>[30x]GAPGAPGSQGAPGLQGAPGAPGSQGAPGLQGAPGAPGSQGAPGLQGAPGAPGSQGAPGLQGAPGAPGSQGAPGLQGAPGAPGSQGAPGLQGAPGAPGSQGAPGLQGAPGAPGSQGAPGLQGAPGAPGSQGAPGLQGAPGA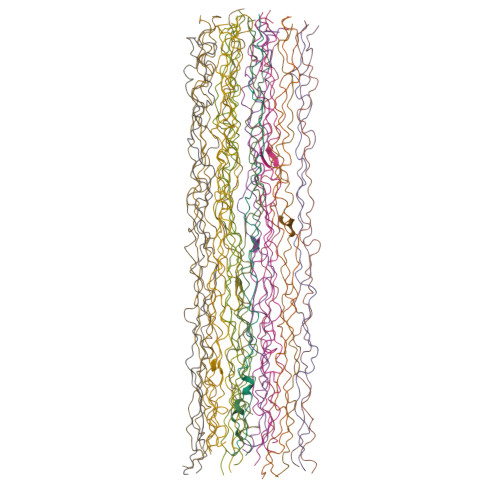PGSQGAPGLQGAPGAPGSQGAPGLQGAPGAPGSQGAPGLQGAPGAPGSQGAPGLQGAPGAPGSQGAPGLQGAPGAPGSQGAPGLQGAPGAPGSQGAPGLQGAPGAPGSQGAPGLQGAPGAPGSQGAPGLQGAPGAPGSQGAPGLQGAPGAPGSQGAPGLQGAPGAPGSQGAPGLQGAPGAPGSQGAPGLQGAPGAPGSQGAPGLQGAPGAPGSQGAPGLQGAPGAPGSQGAPGLQGAPGAPGSQGAPGLQGAPGAPGSQGAPGLQGAPGAPGSQGAPGLQGAPGAPGSQGAPGLQGAPGAPGSQGAPGLQGAPGAPGSQGAPGLQGAPGAPGSQGAPGLQGAPGAPGSQGAPGLQGAPGAPGSQGAPGLQGAPGAPGSQGAPGLQGAPGAPGSQGAPGLQGAPGAPGSQGAPGLQGAPGAPGSQGAPGLQGAPGAPGSQGAPGLQGAPGAPGSQGAPGLQGAPGAPGSQGAPGLQGAPGAPGSQGAPGLQGAPGAPGSQGAPGLQGAPGAPGSQGAPGLQGAPGAPGSQGAPGLQGAPGAPGSQGAPGLQGAPGAPGSQGAPGLQGAPGAPGSQGAPGLQGAPGAPGSQGAPGLQGAPGAPGSQGAPGLQGAPGAPGSQGAPGLQGAPGAPGSQGAPGLQ>MKSVVNDTDGIVRVAESVIPEIKHQDEVRVKIASSGLCGSDLPRIFKNGAHYYPITLGHEFSGYIDAVGS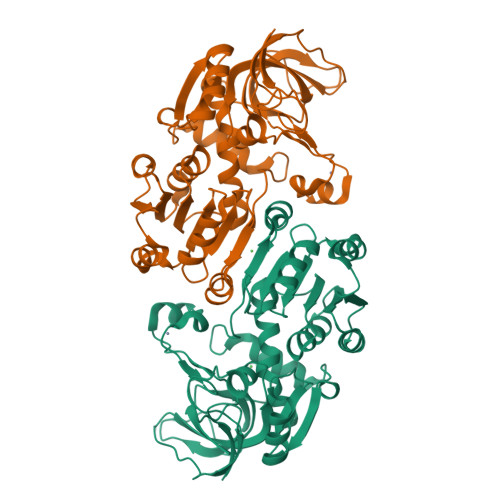GVDDLHPGDAVACVPLLPCFTCPECLKGFYSQCAKYDFIGSRRDGGFAEYIVVKRKNVFALPTDMPIEDGAFIEPITVGLHAFHLAQGCENKNVIIIGAGTIGLLAIQCAVALGAKSVTAIDISSEKLALAKSFGAMQTFNSSEMSAPQMQSVLRELRFNQLILETAGVPQTVELAVEIAGPHAQLALVGTLHQDLHLTSATFGKILRKELTVIGSWMNYSSPWPGQEWETASRLLTERKLSLEPLIAHRGSFESFAQAVRDIARNAMPGKVLLIP[2x]>MQKTLEVWIMPNSPQPAEDFKALVAPFEKAHGVEVKVTVLDWGVAWTKITTAATSGVGPDLTQLGTTWVGAISAMGVLEPVDDVLEALGGEKAYLPAVWRTTRLEGARQATAVPWFSELRAFYYRTDALKAAGVNPAEMFASWQGFEAGLARLKASSFRDPETKAPLAPLCTPGRTPRTLHNAAPWIWGAGGEIVRQAGGRWQSALNSPESLEGLYFFLSLAQKGYVPAESLEKNTAQIEADFQAGKCAVFASGP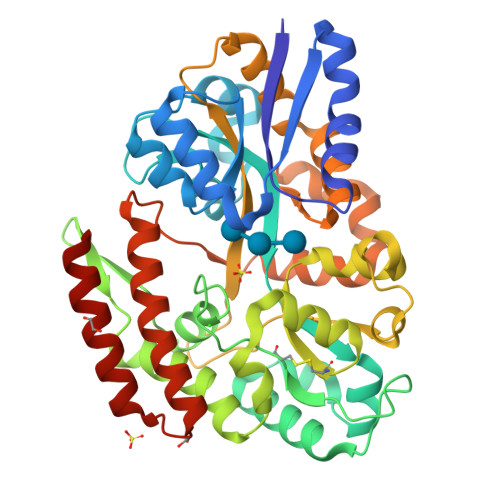WMIQRAQVPEAKGGFAERTAAKNLGVAPYPAGPKGRYTFFGGSNLALFNFSKNKPLAKELLKYLGGPEAQVRYAQMTGMLPALRSAWSDPSFQQNPLLRTFIQAAQFGRTYPSLAGWGGVENLAVQHLGMAWDLVAQGRLTREALKDLMDKASAAINQALRHHHHHH[3x]>SWQTYVDEHLMCDIDGQGQQLAASAIVGHDGSVWAQSSSFPQFKPQEITGIMKDFEEPGHLAPTGLHLGGIKYMVIQGEAGAVIRGKKGSGGITIKKTGQALVFGIYEEPVTPGQCNMVVERLGDYLIDQGL[2x]

Bet v 2 is a plant profilin panallergen, i.e., it is ubiquitously distributed throughout nature and shares a highly conserved amino acid sequence of up to 75% even between distantly-related organisms. Additionally to its ability to bind actin, profilins also interact with poly-l-proline and phosphoinositides. In this study, we present crystal structures of Bet v 2 in the reduced (without disulfide bridge) and the oxidized (with disulfide bridge) states at a resolution of 2.0 and 1.7 Å respectively. The reduced and oxidized structures were determined at a high resolution of 2.0 Å and 1.7 Å, respectively. Both structures share a central six-stranded antiparallel β-sheet with two N- and the C-terminal α-helices flanking the sheet at one side and a third helix flanking the sheet on the opposite side.

While the overall structure was conserved between these two forms, the crystal structures revealed marked differences near the N- and C-terminal segments, which are linked by the disulfide bridge Cys13-Cys117. By contrast, in the reduced form the helix is more relaxed and extends beyond Cys117, which is rotated by approximately 30° between the oxidized and reduced structures. Moreover, the N-terminal segment harboring Cys13 was moved away from the helix for approximately 13 Å and is partially disordered. In fact, Cys13 is visible in the electron density only in one of the two molecules within the asymmetric unit, and Asp14 to Gln21 is disordered in both molecules of the asymmetric unit. The higher degree of disorder in the reduced form, lacking a disulfide bridge, is also reflected in the overall Cα-rmsd of 0.744 Å between the two molecules in the asymmetric unit of the reduced Bet v 2 crystal. To test the secondary structure content, we pursued CD and FTIR spectroscopy. Both methods revealed a slight increase of helical content in the reduced Bet v 2 form as compared to the oxidized form. Importantly, cathepsin S showed a strong preference for the reduced Bet v 2 isoform, which was completely degraded after 10 min. The reduced form of Bet v 2 was found prone to dimerization and higher oligomerization states under non-reducing conditions, whereas the oxidized form of Bet v 2 remained stable as a monomer. This can be explained by the exposed cysteine 13 in the reduced Bet v 2 crystal structure.> MAAQPPRGIRLSALCPKFLHTNSTSHTWPFSAVAELIDNAYDPDVNAKQIWIDKTVINDHICLTFTDNGNGMTSDKLHKMLSFGFSDKVTMNGHVPVGLYGNGFKSGSMRLGKDAIVF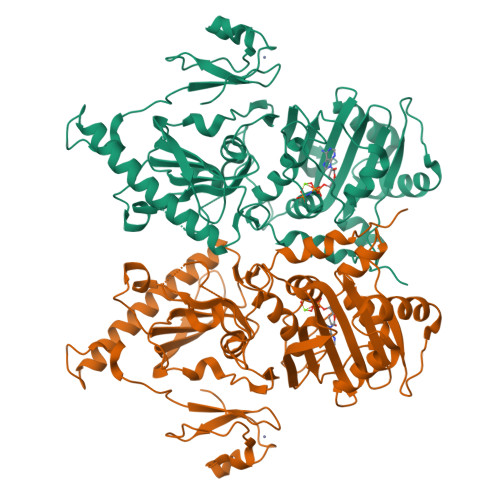TKNGESMSVGLLSQTYLEVIKAEHVVVPIVAFNKHRQMINLAESKASLAAILEHSLFSTEQKLLAELDAIIGKKGTRIIIWNLRSYKNATEFDFEKDKYDIRIPEDLDEITGKKGYKKQERMDQIAPESDYSLRAYCSILYLKPRMQIILRGQKVKTQLVSKSLAYIERDVYRPKFLSKTVRITFGFNCRNKDHYGIMMYHRNRLIKAYEKVGCQLRANNMGVGVVGIIECNFLKPTHNKQDFDYTNEYRLTITALGEKLNDYWNEMKVKKNTEYPLNLPVEDIQKRPDQTWVQCDACLKWRKLPDGMDQLPEKWYCSNNPDPQFRNCEVPEEPEDE> MHLNPAEKEKLQIFLASELALKRKARGLKLNYPEAVAIITSFIMEGARDGKTVAMLMEEGKHVLTRDDVMEGVPEMIDDIQAEATFPDGTKLVTVH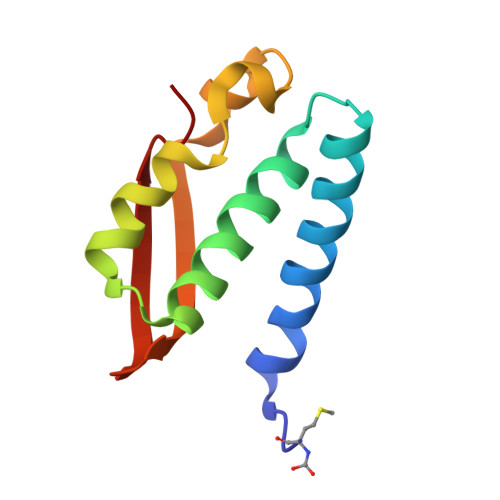NPIS>MSNSAKSPSGPVGDEGRRNYPMSAHTLVTQEQVWAATAKCAKKIAEDYRSFKLTTDNPLYLLCVLKGSFIFTADLARFLADEGVPVKVEFICASSYGTGVETSGQVRMLLDVRDSVENRHILIVEDIVDSAITLQYLMRFMLAKKPASLKTVVLLDKPSGRKVEVLVDYPVITIP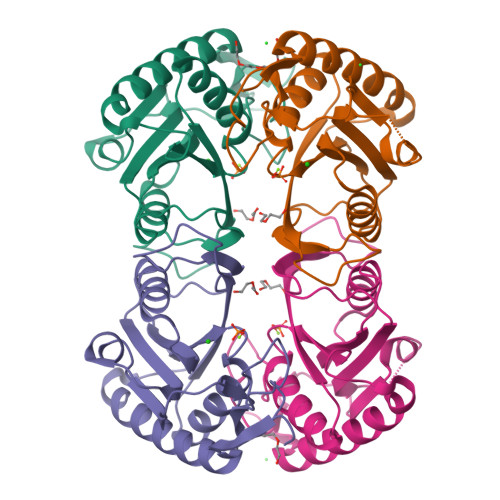HAFVIGYGMDYAESYRELRDICVLKKEYYEKPESKV[2x]> CGCUUCAUAUAAUCCUAAUGAUAUGGUUUGGGAGUUUCUACCAAGAGCCUUAAACUCUU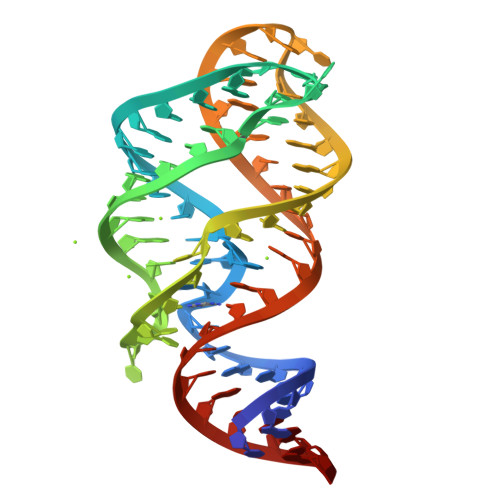GAUUAUGAAGUG> GSHMGQELVSLEGHQSAITALAFSKNIVVSGAADGTIKVWDILTGQLLRDHDGHQSEVTALQFKDNIVVSGAKDGTVKVWYIGTGQELVSLEGHQSAITALAFSKNIVVSGAADGTIKVWDILTGQLLRDHDGHQSEVTALQFKDNIVVSGAKDGTVKVWYIGTGQELVSLEGHQSAIT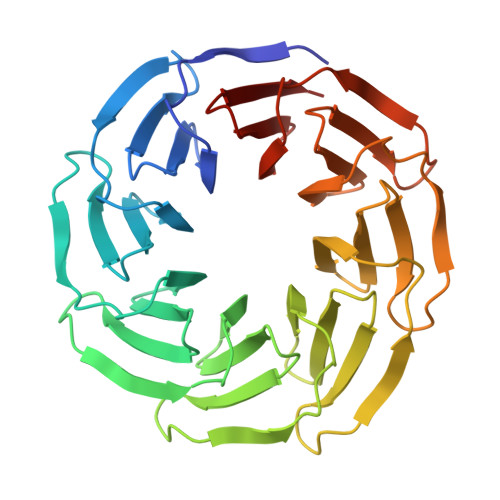ALAFSKNIVVSGAADGTIKVWDILTGQLLRDHDGHQSEVTALQFKDNIVVSGAKDGTVKVWYIGTGQELVSLEGHQSAITALAFSKNIVVSGAADGTIKVWDILTGQLLRDHDGHQSEVTALQFKDNIVVSGAKDGTVKVWYIGT>MHHHHHHHHHHGTETVRFQSKQNNNFSVRALPSFIDVFNGIYGFATGIQDIFNMIFGTDTGDLTLEEVLKNQELLYDISGKLEGISGDLSEIIAQGNLNTELAKELLKIANEQNNVLTDVNNKLNAINSMLHIYLPKITNMLSDVMKQNYALSLQIEYLSKQLQEISDKLDVINLNVLINCTCTEITPAYQRIKYVNEKFDELTLATEKTLRAKQGSEDIIANDTLENLTELTELAKSVTKNDMDSFEFYLHTFHDVLIGNNLFGRSALKTAAELITKDEIKTSGSEIGKVYSFLIVLTCLQAKAFLTLTACRKLLGLSDIDYTNILNQHLNDEKNVFRDNILPTLSNKFSNPNYVKTIGSDNYAKVILEAEPGYALVGFEIINDRIPVLKAY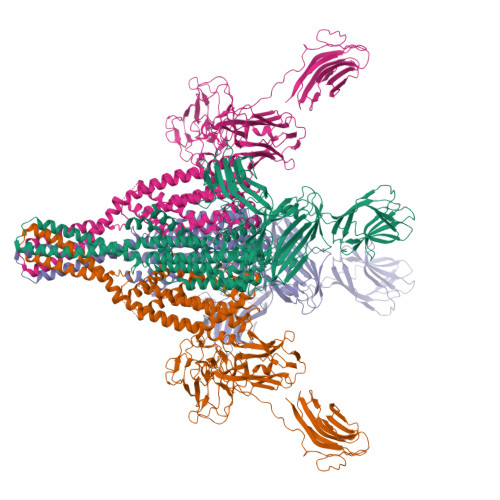KAKLKQNYQVDHQSLSEIVYLDIDKLFCPKNSEQKYYTKSLTFPDGYVITKITFEKKLNNLRYEATANFYDPSTGDIDLNEKQVESTFLQADYISINVSDDDGVYMPLGVISETFLSPINSFELEVDEKSKILTLTCKSYLREYLLESDLINKETSLIAPPNVFISNIVENWNIEADNLEPWVANNKNAYVDSTGGIEGSKALFTQGDGEFSQFIGDKLKPNTDYIIQYTVKGKPAIYLKNKNTGYTMYEDTNGSSEEFQTIAVNYTSETDPSQTHLVFKSQSGYEAWGDNFIILECKAFETPEGPELIKFDDWISFGTTYIRDDVLTIDPSRGGYFRQSLKLDSYSTYNLSFSFSGLWAKVIIKNSHGVVLFEKVSQQSSYVDISESFTTTSNKEGFFIELTGDSRGGFGSFRDFSMKEKFE[4x]>[2x]DYKDDDDKVKLYK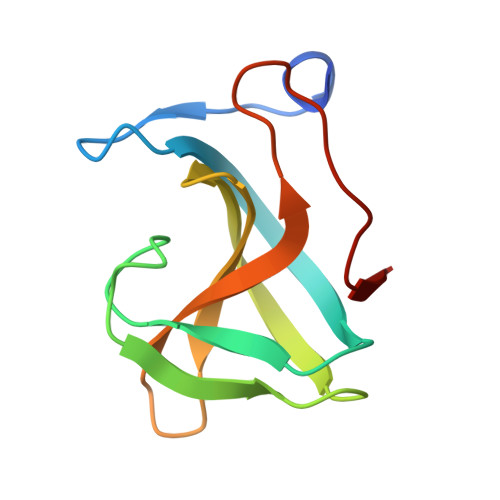TNKYGTLYKSESASFTANTDIITRLTGPFRSMPQSGVLRKGLTIKYDEVMKQDGHVWVGYNTNSGKRVYLPVRTWNESTGELGPLWGTIK>[2x]MHHHHHHMKSYFVTMGFNETFLLRLLNETSAQKEDSLVIVVPSPIVSGTRAAIESLRAQISRLNYPPP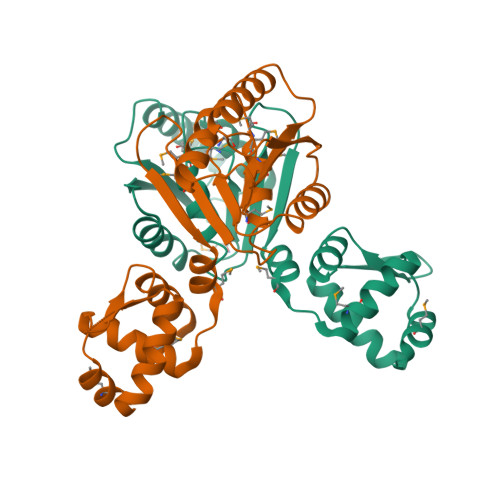RIYEIEITDFNLALSKILDIILTLPEPIISDLTMGMRMINTLILLGIIVSRKRFTVYVRDEGGGSRVISFNDNTIRALMRDYSREEMKLLNVLYETKGTGITELAKMLDKSEKTLINKIAELKKFGILTQKGKDRKVELNELGLNVIKLNKSVIESSKSSEELVKENKGKEVNIPY> MASVHGTTYELLRRQGIDTVFGNPGSNELPFLKDFPEDFRYILALQEACVVGIADGYAQASRKPAFINLHSAAGTGNAMGALSNAWNSHSPLIVTAGQQTRAMIGVEALLTNVDAANLPRPLVKWSYEPASAAEVPHAMSRAIHMASMAPQGPVYLSVPYDDWDKDADPQSHHLFDRH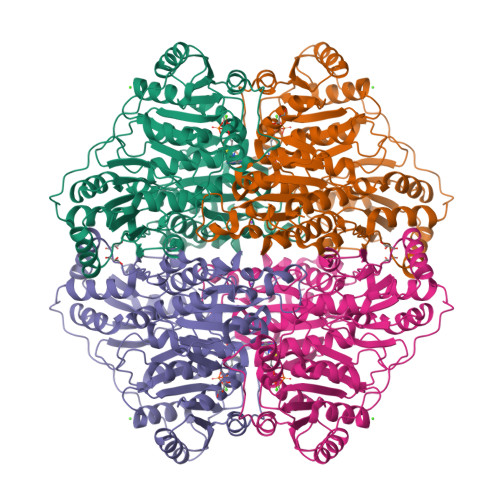VSSSVRLNDQDLDILVKALNSASNPAIVLGPDVDAANANADCVMLAERLKAPVWVAPSAPRCPFPTRHPCFRGLMPAGIAAISQLLEGHDVVLVIGAPVFRYHQYDPGQYLKPGTRLISVTCDPLEAARAPMGDAIVADIGAMASALANLVEESSRQLPTAAPEPAKVDQDAGRLHPETVFDTLNDMAPENAIYLNESTSTTAQMWQRLNMRNPGSYYFCAAGGFGFALPAAIGVQLAEPERQVIAVIGDGSANYSISALWTAAQYNIPTIFVIMNNGTYGALRWFAGVLEAENVPGLDVPGIDFRALAKGYGVQALKADNLEQLKGSLQEALSAKGPVLIEVSTVSPVKRSHHHHHH>[2x]GHMKISWNGFSKKSYQERLELLKAQALLSPERQASLEKDEQMSVTVADQLSENVVGTFSLPYSLVPEVLVNGQEYTVPYVTEEPSVVAAASYASKIIKRAGGFTAQVHQRQMIGQVALYQVANPKLAQEKIASKKAELLELANQAYPSIVKRGGGARDLHVEQIKGEPDFLVVYIHVDTQEAMGANMLNTMLEALKPVLEELSQGQSLMGILSNYA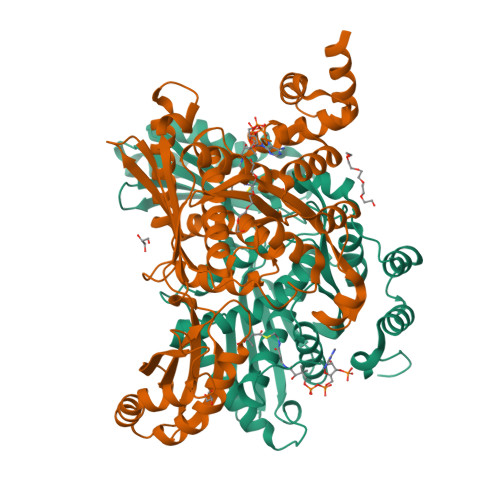TDSLVTASCRIAFRYLSRQKDQGREIAEKIALASQFAQADPYRAATHNKGIFNGIDAILIATGNDWRAIEAGAHAFASRDGRYQGLSCWTLDLEREELVGEMTLPMPVATKGGSIGLNPRVALSHDLLGNPSARELAQIIESIGLAQNFAALKALVSTGIQQGHMKLQAKSLALLAGASESEVAPLVERLISDKTFNLETAQRYLENLRS> MEPD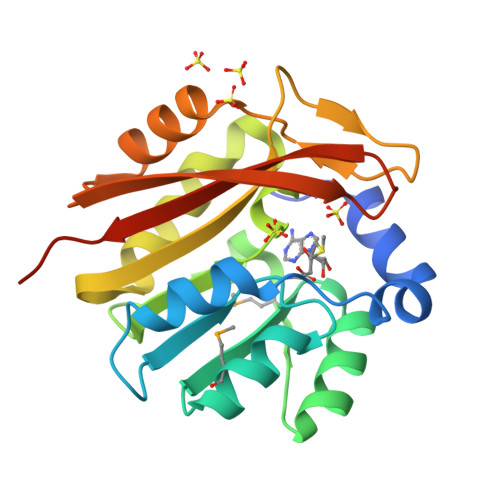MTQAFDDDTLRFYRGNATAYAERQPRSATLTKFLGELPAGAKILELGCGAGYQAEAMLAAGFDVDATDGSPELAAEASRRLGRPVRTMLFHQLDAIDAYDAVWAHACLLHVPRDELADVLKLIWRALKPGGLFYASYKSGEGEGRDKLARYYNYPSEEWLRARYAEAGTWASVAVESSEGKGFDQELAQFLHVSVRKPELEHHHHHH> GHMMKNRIFVSSSKDFEGYPSKAIVPVQFVALLTSIHLTETKCLLGFSNFERRGDQSQEDQYLIKLKFKDRGSERLARITISLLCQYFDIELPDLDSDSGASPTVILRDIHLERLCFSSCKALYVSKHGNYTLFLEDIKPLDLVSVISTISTKSTNSSKHSSSELISECDLNNSLVDIFNNLIEMNRDEKNRFKFV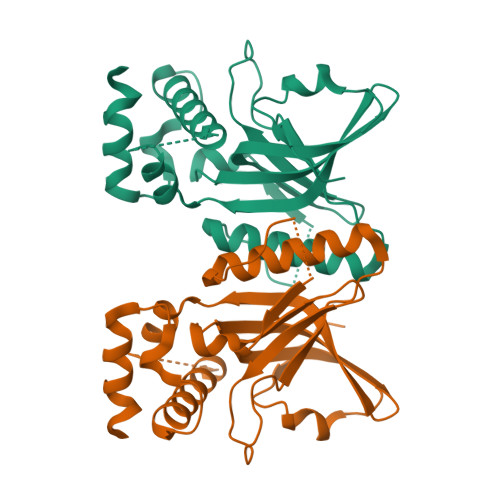KLIHYDIELKKFVQDQQKVLSQK>SFAPGMVSQKCLLCMCKLESGGCKPIGCRMDVGSLSCGYFQIKQPYWIDCGKPGKDWKSCS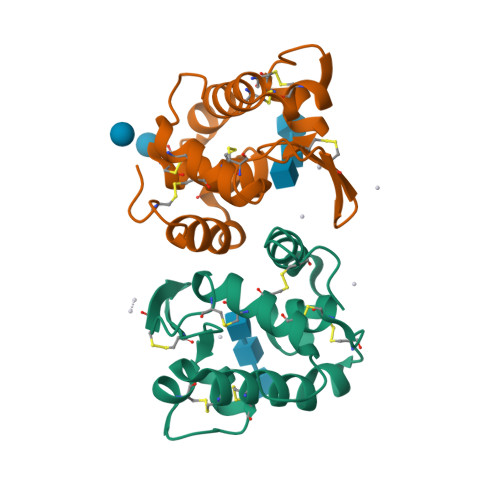NDINCSSKCVQQYMKRYATHYRCPLNCEGFAREHNGGPNGCHSSRTLKYWELLQKIPGCKGVK[2x]>MSLLLTNHIGYERLGPKKAIIQTEQPHLSSYTAQLICATSEQTVATFAVEEQGKVANWHQGYFYLIDFSSFTDSGDYFLQVEDSRSSTFTVGEHILLNQTLSDVIHYFKSQRCGGVFDQQDRQVPVLNANQTADVHGGWYDASGDVSKYLSHLSYANYLNPQQTPMVVWNILKGLSLLEGSEDIAAFTRTRLIEEALFGADFLVRMQNEKGFFYMTVFDKWSKDTAQREICAYETQLGHKFDDYQAGFRQGGGVAIAALAAASRLGVHGEYDQQKYRNAAENGYWHLKEHNTQYLNDGEENIIDEYCALLASVELFKATKETRYLEESRLWAQRLVARQMSDEQIQHFWSANQDGSRPYFHAAEAGLPTIALCEYLAIEDDSVQTESVKCIVNRACEFEIKISNKVTNPFGYPRQYVKGVNESKRDAFFVAHNNESGYWWQGENARLGSLATMAYLAQPHIASQEIQQQLSVFAQDALNWIVGLNPYDMCMLDGHGRNNPDYLPQYGFFNAKGGVCNGITGGFEDEEDIAFNPPAQKDDMLQNWRWGEQWIPHGAWYLLAIMSQAQHISQLATSKNIKEGHHHHHH[3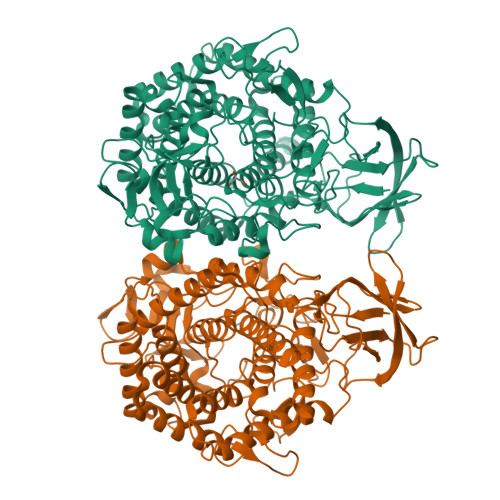x]> GHMSHLADVSPPTACRVCGGGVQEFLDLGRQPLSDRFRKPDELDDEFTYRLAVGRCDSCEMVQLTEEVPRDLMFHEVFPYHSSGSSVMREHFAMLARDFLATELTGPDPFIVEIGCNDGIMLRTIQEAGVRHLGFEPSSGVAAKAREKGIRVRTDFFEKATADDVRRTEGPANVIYAANTLCHIPYVQSVLEGVDALLAPDGVFVFEDPYLGDIVAKTSFDQIYDEHFFLFSATSVQGMAQRCGFELVDVQRLPVHGGEVRYTLARQGS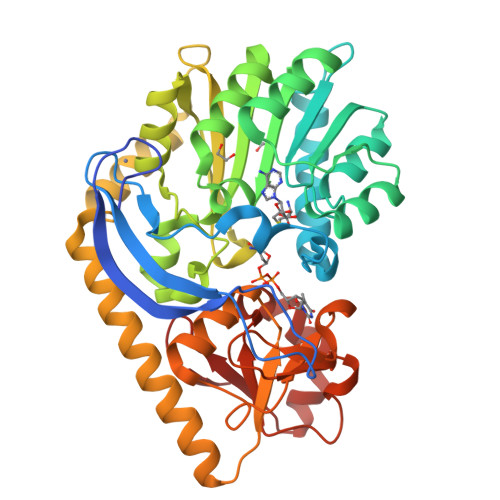RTPSAAVAQLLAAEREQELSDMATLRAFAGNVVKIRDELTALLHRLRAEGRSVVGYGATAKSATVTNFCGIGPDLVHSVYDTTPDKQNRLTPGAHIPVRPASAFSDPYPDYALLFAWNHAEEIMAKEQEFHQAGGRWILYVPEVHIR> MTMLGERLVLRWRVAASFAWSVILMPVCCALFIVLSRIQILHPIQWLTDSISDLTSSYTIFCLLLICAILGLQCTFLMEYYTVVPSIPCSRLALIGNLLLPHRILHSLAHVAMGVLASWCYAVLSKGKYQLLVVSCTLQSEDEADKPSHCLNESHLFQLLCGAFFGYSYSLQYFVHNMNYLSFPSIQQYKYLQFRRFLPLIIKQSVFQSLYFIRSYAILYFCLGNIPRTWIQTALNLHMDRQQPSLDTLRGFLNLSLFYQIWLSGTFLLATWYMVWILFRIYTTEARIFPVQTSFAEEAEKCLPFILNSNTLPLVKYLAMQDLVLLSQYSPSRRQEVFSLSQPGGHPHNWTSISKECLNLMSSLTSRLIAHQEAAANNGRMRVPSSPKQIRKS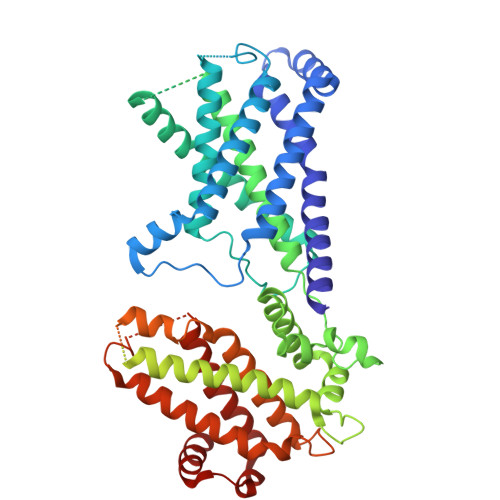SSSSGTSLIEDSAEQTQNLSTIPRIGIPSLLKTASLKSSLDIGSPFATPGVKQMSESLDPNTPCHGSVQSPQVTRRGAKLWTSDSDVQKNGSEVSPVMHRPVCNGAKQGILHTWFQHKLVQIKNVLSKRGLIMYLFSKHPEASSQDVFADAQIHIWALEALSHLVAASFSEDRMGVVQTSLSSVLAILLTLQEAVEKHFKLPHASSKPARNPGSLLDSSCKTLRFSLRAALKTAIYRITTTFGEHLHAVPVSSEHKKKLQQFLDFKE> GAMESKKRQWALEDFEIGRPLGKGKFGNVYLAREKQSKFILALKVLFKAQLEKAGVEHQLRREVEIQSHLRHPNILRLYGYFHDATRVYLILEYAPLGTVYRELQKLSKFDEQRTATYITELANALSYCHSKRVIHRDIKPENLLLGSAGELKIADFGWSVHAPSSRRTTLAGTLDYLPPEMIEGRMHDEKVDLWSLGVLCYEFLVGKPPFEANTYQETYKRISRVEFTFPDFVTEGARDLISRLLKHNPSQRPMLREVLEHPWITANSSKPSNAQNKESASKQS

Over the last decade, extensive research has been directed towards the discovery of small molecule inhibitors of the Aurora protein kinases as anticancer agents. We have previously reported imidazo[4,5-b]pyridine-based inhibitors of Aurora kinases including 1 (CCT137690),10 the dual FLT3/Aurora kinase inhibitor 2 (CCT241736),11 and compound 3 which selectively inhibits Aurora-A over Aurora-B12. Introduction of a 1-benzyl-1H-pyrazol-4-yl moiety at C7 of the imidazo[4,5-b]pyridine scaffold provided 7a which inhibited a range of kinases including Aurora-A. Modification of the benzyl group in 7a, and subsequent co-crystallisation of the resulting analogues with Aurora-A indicated distinct differences in binding mode dependent upon the pyrazole N-substituent. In addition, we report ligand/Aurora-A protein crystallographic data that show different orientations for the substituent on the pyrazole ring suggesting that the 7-(pyrazol-4-yl)-3H-imidazo[4,5-b]pyridine scaffold could be utilised for the design of compounds that additionally interact with the DFG motif or with Thr217, the latter tactic has been demonstrated to enhance Aurora-A over Aurora-B selectivity.

As part of our medicinal chemistry programme to discover selective inhibitors of Aurora-A,12 we introduced the 1-benzyl-1H-pyrazol-4-yl moiety at C7 of the imidazo[4,5-b]pyridine scaffold to provide 7a. In biochemical assays, 7a inhibited both Aurora-A and Aurora-B with IC50 values of 0.212 and 0.461 μM, respectively. To understand the potential for further improvement, we obtained the crystal structure of 7a bound to Aurora-A22. This structure shows the ligand in the ATP binding site with the pyridine nitrogen atom hydrogen bonded to the backbone NH of Ala213 and the imidazole NH interacting with the carbonyl of Ala213, consistent with previous reports of the hinge binding mode for the imidazo[4,5-b]pyridine scaffold. Similar to crystal structures of previous compounds 1, 15 and 16 (compounds 51 and 40c in Ref. 10, and compound 21a in Ref. 11, respectively) the N-benzyl substituent on the C7-pyrazole is oriented towards the P-loop, making Van der Waals contacts with Val147 and Gly142. In an attempt to improve the aqueous solubility, the Aurora inhibitory potency and kinase selectivity of this sub-series, we explored the introduction of basic substituents such as 1-methylpiperazine and pyrrolidine as well as replacement of the phenyl ring with a more polar heterocycle. This approach was guided by the ligand/protein interactions observed in the protein crystal structure of 7a, which showed that the N-benzyl substituent on the C7-pyrazole is oriented towards the P-loop. Compounds 7a and 14d interact with the P-loop whereas 14a and 14b engage with Thr217 in the post-hinge region.>[2x]GSHGGSMKAANASSAEAYRVLSRAFRFDNEDQKLWWHSTAPMFAKMLETANYTTPCQYQYLITYKECVIPSLGCYPTNSAPRWLSILTRYGTPFELSLNCSNSIVRYTFEPINQHTGTDKDPFNTHAIWESLQHLLPLEKSID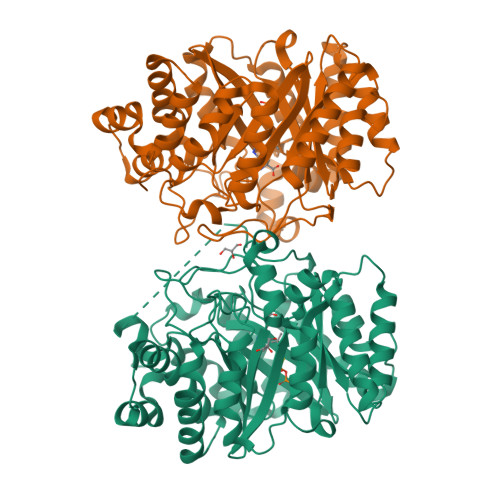LEWFRHFKHDLTLNSEESAFLAHNDRLVGGTIRTQNKLALDLKDGRFALKTYIYPALKAVVTGKTIHELVFGSVRRLAVREPRILPPLNMLEEYIRSRGSKSTASPRLVSCDLTSPAKSRIKIYLLEQMVSLEAMEDLWTLGGRRRDASTLEGLSLVRELWDLIQLSPGLKSYPAPYLPLGVIPDERLPLMANFTLHQNDPVPEPQVYFTTFGMNDMAVADALTTFFERRGWSEMARTYETTLKSYYPHADHDKLNYLHAYISFSYRDRTPYLSVYLQSFETGDWAVANLSESKVKCQDAACQPTALPPDLSKTGVYYSGLH> AFVVTDNCIKCKYTDCVEECPVDCFYEGPNFLVIHPD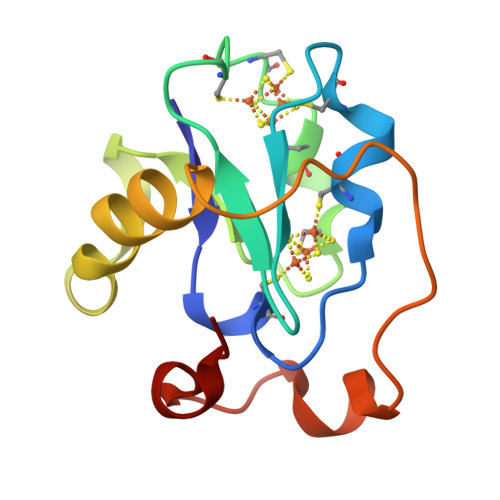ECIDCALCEPECPAQAIFSEDEVPEDMQEFIQLNAELAEVWPNITEKKDPLPDAEDWDGVKGKLQHLER> MVDYRVVFHIDEDDESRVLLLISNVRNLMADLESV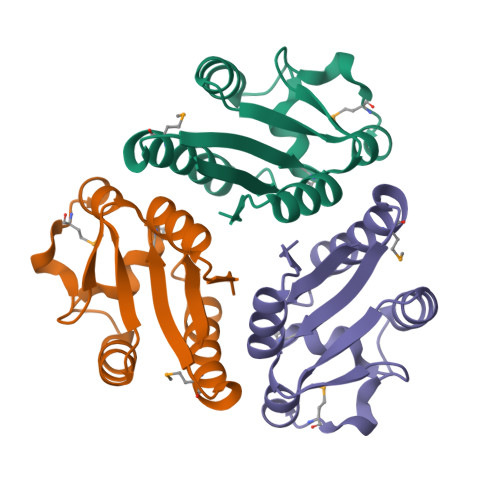RIEVVAYSMGVNVLRRDSEYSGDVSELTGQGVRFCACSNTLRASGMDGDDLLEGVDVVSSGVGHIVRRQTEGWAYIRP>[2x]SNAMIKRPIHMSHDFLAEVLDDESIVVDATMGNGNDTAFLAGLSKKVYAFDVQEQALGKTSQRLSDLGIENTE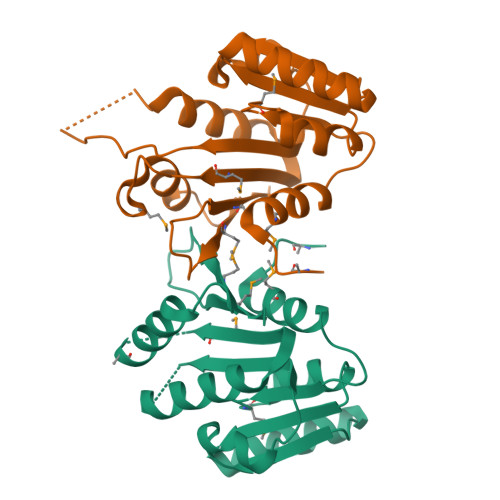LILDGHENLDHYVREPIRAAIFNLGYLPSADKSVITKPHTTLEAIEKILDRLEVGGRLAIMIYYGHDGGDMEKDAVLEYVIGLDQRVFTAMLYQPLNQINTPPFLVMLEKLQ>[2x]AVEQCDLSQFQTTSSNQLMAAIRQQGASCVNALFSADTGVQEAAFSSNHMYNVAQYTRTLAQQYAGGGSDELEALYLYLRAGYYAEFYNSNITFLSWVTPAVKGAVDAFVQNAHFYDNGDAHGKVLNEVIITMDSAGLQHAYLDVVTQWLTRWNAQYAEHWYMRNAVNGVFTLLFGGQWNNQYTSLIGEQTALVTALQAFALDRTKVNSPTEFMAANAARELGRLARYTDATIAPKVTEGLTAIFGQYPSYGDGDAIWLGAADTASYYADCSQFNICGFEDALRDAALNQTFICSDTIKIRSQDMSQAQHLAACDKMAYEESFFHTTLETGNQPVADDHNTQLQVNIFNSDTDYGKYAGPIFGIDTNNGGMYLEGNPANVGNIPNFIAYEASYANPDHFVWNLEHEYVHYLDGRFNMYGDFGTPTELVVWWSEGVAEYVSRVNDNPQAIATIQDGSTYTLAQVFDTTYDGFDVDRIYRWGYLAVRFMFERHPDEVQRMLSATRQGRWAEYKAIISGWANQYQSEFAQWTEALAKGDSGAGNGEGTGSGNEGGGESGGNT

Collagenase from the gram-negative bacterium Grimontia hollisae strain 1706B (Ghcol) degrades collagen more efficiently even than clostridial collagenase, the most widely used industrial collagenase. Collagenase (Enzyme Commission number: 3.4.24.3) cleaves the triple-helical region of collagen under physiological conditions, catalyzing the hydrolysis of peptide bonds with glycine residues at the P1 position. It produces the collagenase Ghcol, which consists of 767 amino acid residues with a single catalytic domain containing the zinc-binding motif H492EYVH496. Here, we report the crystal structures of ligand-free and Gly-Pro-hydroxyproline (Hyp)-complexed Ghcol at 2.2 and 2.4 Å resolution, respectively. These structures revealed that the activator and peptidase domains in Ghcol form a saddle-shaped structure with one zinc ion and four calcium ions.

To obtain a homogeneous preparation, we expressed the collagenase module (Ala88–Thr646) of Ghcol with the Sec signal peptide using the B. chosinensis expression system and purified it from the supernatant. Crystals of ligand-free Ghcol were obtained. The space groups of ligand-free and ligand-complexed Ghcol structures are C2 and P21, respectively. Both crystals contain two molecules (chains A and B) in the asymmetric unit of the cell. In addition, the activator domain comprises two homologous subdomains, whereas zinc-bound water was observed in the ligand-free Ghcol. The structure is divided into the activator domain (Ala88–Tyr355), linker (Ala356–Gly365), and peptidase domain (Phe366–Gly622). The peptidase domain is further divided into two subdomains, namely the upper half (C1: Phe366–Val515) and lower half (C2: Val516–Gly622). Comparison of the zinc-binding motifs of Ghcol and ColG revealed that both contain two His residues (His492 and His496 for Ghcol and His523 and His527 for ColG) and one Glu residue (Glu520 for Ghcol and Glu555 for ColG) that coordinate to the zinc ion, and the catalytic Glu residue and one water molecule are located near the zinc ion. In this study, the overall structures of Ghcol and ColG are shown to be similar with an RMSD of 1.56 to 2.38 Å.>MKKIFMMVHELDVNKGGMTSSMFNRSKEFYDADIPADIVTFDYKGNYDEIIKALKKQGKMDRRTKMYNVFEYFKQISNNKHFKSNKLLYKHISERLKNTIEIEESKGISRYFDITTRTYIAYIRKSKSEKVIDFFKDNKRIERFSFIDNKVHMKETFNVDNKVCYQVFYDEKGYPYISRNINANNGAVGKTYVLVNKKEFKNNLALCVYYLEKLIKDSKDSIMICDGPGSFPKMFNTNHKNAQKYGVIHVNHHENFDDTGAFKKSEKYIIENANKINGVIVLTEAQRLDILNQFDVENIFTISNFVKIHNAPKHFQTEKIVGHISRMVPTKRIDLLIEVAEL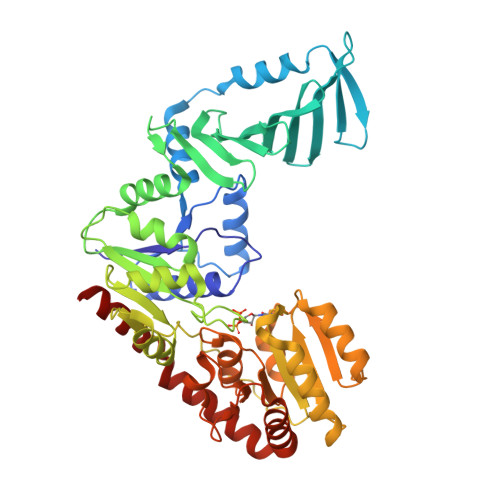VVKKDNAVKFHIYGEGSVKDKIAKMIEDKNLERNVFLKGYTTTPQKCLEDFKLVVSTSQYEGQGLSMIEAMISKRPVVAFDIKYGPSDFIEDNKNGYLIENHNINDMADKILQLVNNDVLAAEFGSKARENIIEKYSTESILEKWLNLFNS[2x]>GHMKTNPIYWKATNPTLSPSHLQDLPGFTRSVYKRDHALITPESHVYSPLPDWTNTLGAYLITPATGSHFVMYLAKMKEM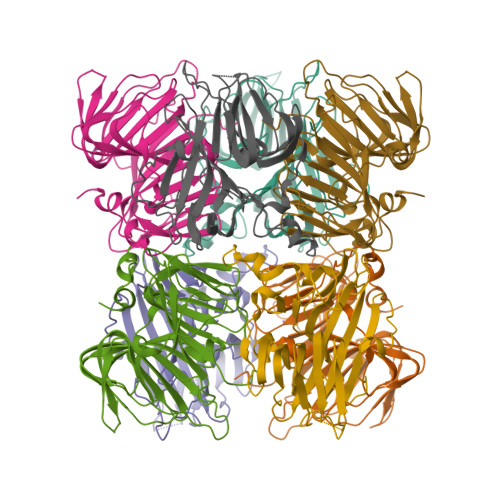SSSGLPPQDIERLIFVVEGAVTLTNTSSSSKKLTVDSYAYLPPNFHHSLDCVESATLVVFERRYEYLGSHTTELIVGSTDKQPLLETPGEVFELRKLLPMSVAYDFNIHTMDFQPGEFLNVKEVHYNQHGLLLLEGQGIYRLGDNWYPVQAGDVIWMAPFVPQWYAALGKTRSRYLLYKDVNRNPL[16x]> PGSMTLSSNQYQLPLNVRPYTTTWCSQSPSCSNLLAIGHDTGITIYCASEEQTPGSTGLTLQELFTIQTGLPTLHLSFSSSCSYSENLHDGDGNVNS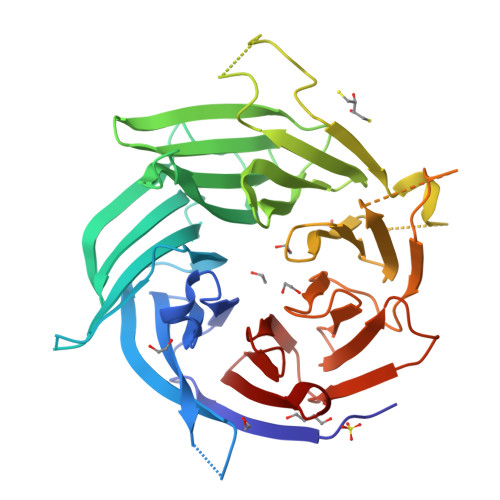SPVYSLFLACVCQDNTVRLIITKNETIITQHVLGGKSGHHNFVNDIDIADVYSADNRLAEQVIASVGDDCTLIIWRLTDEGPILAGYPLSSPGISVQFRPSNPNQLIVGERNGNIRIFDWTLNLSAEENSQTELVKNPWLLTLNTLPLVNTCHSSGIASSLANVRWIGSDGSGILAMCKSGAWLRWNLFANNDYNEISDSTMKLGPKNLLPNVQGISLFPSLLGACPHPRYMDYFATAHSQHGLIQLINTYEKDSNSIPIQLGMPIVDFCWHQDGSHLAIATEGSVLLTRLMGFTRL> MESKVVVPAQGKKITLQNGKLNVPENPIIPYIEGDGIGVDVTPAMLKVVDAAVEKAYKGERKISWMEIYTGEKSTQVYGQDVWLPAETLDLIREYRVAIKGPLTTPVGGGIRSLNVALRQELDLYICLRPVRYYQGTPSPVKHPELTDMVIFRENSEDIYAGIEWKADSADAEKVIKFLREEMGVKKIRFPEHCGIGIKPCSEEGTKRLVRAAIEYAIANDRDSVTLVHMGNIMKFTEGAFKDWGYQLAREEFG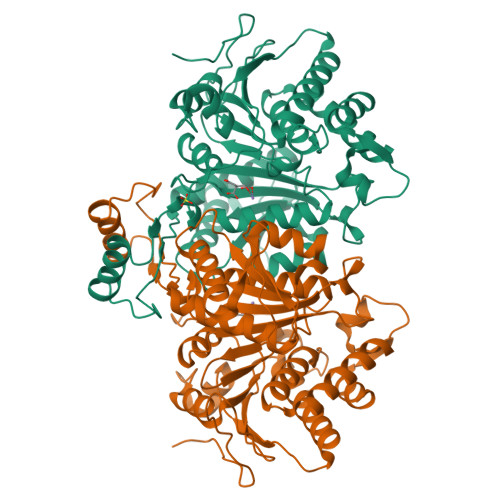GELIDGGPWLKVKNPNTGKEIVIKDVIADAFLQQILLRPAEYDVIACMNLNGDYISDALAAQVGGIGIAPGANIGDECALFEATHGTAPKYAGQDKVNPGSIILSAEMMLRHMGWTEAADLIVKGMEGAINAKTVTYDFERLMDGAKLLKCSEFGDAIIENM> MTSSPATASPAVADQLDSLAALLTSRAQAVRNGAAVPPQQHVQLVKGLKDAAGLVNEAREDLGDLMMSFVQVTALRLLIKWKVFEAIPLEGTISYADVAARVGIDVNLITRLSWVLVATGVLKQDGSDKIQHTARSRPYASRNPLSAMMIIGFDEYLPALLAMPGYFDTYGKKEPFGEKHTVKAFSEGNPELTVNQILASSPERLGNMTLAMAAMENMYPLSGVYDFSWVAAKAASDSNRPLIVDVGGAKGHTLQAICKDTPALPIERCVLEDLPRVIQVVKDTSDAGAQAPQLLGMDFNQEQPVKGAVVYLIRRCLHDYSDEQCVRILGHLAAAMAADS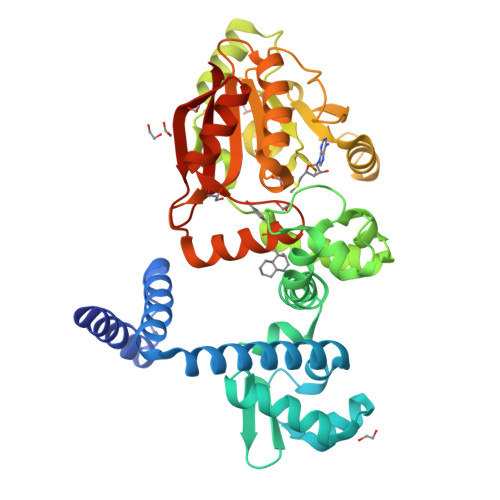VLLIGETVLTNPPSRPTAMMDILLATIGGKERTIDAFGAVVGRAGLRIKGVCKQEGGDFSYIECVKANNNNNN> VVGGTDADEGEWPWQVSLHALGQGHICGASLISPNWLVSAAHCYIDDRGFRYSDPTQWTAFLGLHDQSQRSAPGVQERRLKRIISHPFFNDFTFDYDIALLELEKPAEYSSMVRPICLPDASHVFPAGKAIWVTGWGHTQYGGTGALILQKGEIRVIQQTTCENLLPQQITPRMMCVGFLSGGVDSCQGDSGGPLSSVEADGRIFQAGVVSWGDGCAQRNKPGVYTRLPLFRDWIKENTGV;> QTEDYCLAS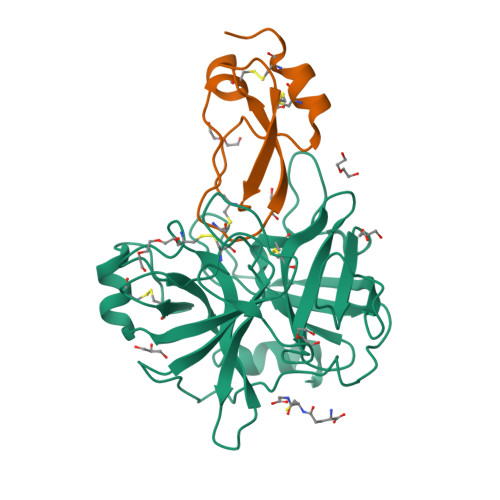NKVGRCRGSFPRWYYDPTEQICKSFVYGGCLGNKNNYLREEECILACRGVQ> SNNKRAPYWTNTEKMEKRLHAVPAANTVKFRCPAGGNPMPTMRWLKNGKEFKQEHRIGGYKVRNQHWSLIMESVVPSDKGNYTCVVENEYGSINHTYHLDVVERSPHRPILQAGLPANASTVVGGDVEFVCKVYSDAQPHIQWIKHVEKNGSKYGPDG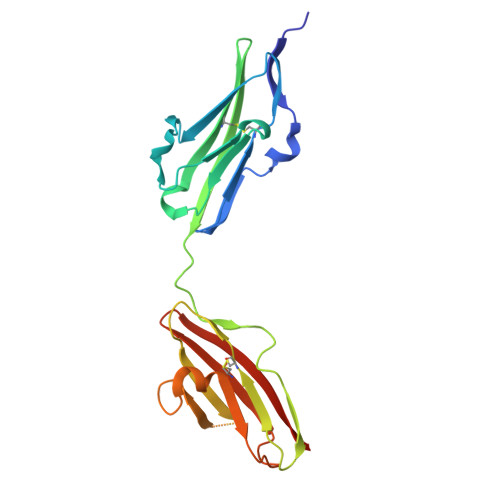LPYLKVLKAAGVNTTDKEIEVLYIRNVTFEDAGEYTCLAGNSIGISFHSAWLTVLPAPGRE Vps34, the primordial phosphatidylinositol 3-kinase (PtdIns3K) that phosphorylates the 3-OH of phosphatidylinositol to form phosphatidylinositol 3-phosphate (PtdIns3P), is conserved in all eukaryotes, and it is important both for endocytic traffic to lysosomes and vacuoles and for autophagy. The minimal Vps34 complex is a heterodimer of Vps34 with Vps15, a putative protein kinase. This Vps34-Vps15 complex is the core for 2 larger, heterotetrameric assemblies known as complexes I and II. In addition to the Vps34-Vps15 core, complex I includes an accessory pair of proteins, Vps30/Atg6 (BECN1 in mammals) and Atg14 (ATG14 in mammals).

The domain organization of Atg38 and NRBF2 sheds some light on how these proteins might function. Both Atg38 and NRBF2 have an N-terminal microtubule-interacting and targeting (MIT) domain and a C-terminal region of unknown structure. We obtained crystals using full-length Atg38 S. cerevisiae protein that had been subjected to limited proteolysis with subtilisin. The structure was solved by multiwavelength anomalous dispersion (MAD) using selenomethionine-derivatized protein and was refined to 2.2 Å resolution. The structure showed that the crystallized region corresponds to residues 119 to 211 in the Atg38 C-terminal domain. The asymmetric unit has 3 copies of an Atg38 homodimer. The ordered parts of the monomers are entirely helical, with a short N-terminal helix A (residues 129 to 150) folded back over a part of a longer helix B (residues 164 to 211). Each homodimer is strikingly asymmetric with the long helix B in one monomer almost straight, while helix B in the other monomer is bent at residue F182 at an angle of approximately 40°. The parallel arrangement of the 2 molecules in a dimer gives rise to a 4-helix bundle at the N-terminal end of the dimer and a long, parallel coiled-coil at the C-terminal end, imparting on the dimer the overall look of a mushroom. We will refer to the segment of the homodimer corresponding to the 4-helix bundle as the cap and the protruding coiled-coil as the stalk and the disordered residues 212 to 226 as the C-terminal tail. Overall, there are 2 homodimerization interfaces in the C-terminal region, one in the cap segment and the other in the stalk segment, both of which we found are important for efficient homodimerization in vivo (see below). The structure of the C-terminal region from Atg38 clearly shows the role of this domain in forming a parallel homodimer.

>MSTLAEVYTIIEDAEQECRKGDFTNAKAKYQEAIEVLGPQNENLSQNKLSSDVTQAIDLLKQDITAKIQELELLIEKQSSEENNIGMVNNNMLIGSVILNNKSPINGISNARNWDNPAYQDTLSPINDPLLMSILNRLQFNLNNDIQLKTEGGKNSKNSEMKINLRLEQFKKELVLYEQKKFKEYGMKIDEITKENKKLANEIGRLRERWDSLVESAKQRRDKQKN[12x]>MNNPAIKRIGNHITKSPEDKREYRGLELANGIKVLLISDPTTDKSSAALDVHIGSLSDPPNIAGLSHFLQHMLFLGTKKYPKENEYSQFLSEHAGSSNAFTSGEHTNYYFDVSHEHLEGALDRFAQFFLSPLFDESAKDREVNAVDSEHEKNVMNDAWRLFQLEKATGNPKHPFSKFGTGNKYTLETRPNQEGIDVRQELLKFHSAYYSSNLMAVVVLGRESLDDLTNLVVKLFSEVENKNVPLPEFPEHPFQEEHLKQLYKIVPIKDIRNLYVTFPIPDLQKYYKSNPGHYLGHLIGHEGPGSLLSELKSKGWVNTLVGGQKEGARGFMFFIINVDLTEEGLLHVEDIILHMFQYIQKLRAEGPQEWVFQELKDLNAVAFRFKDKERPRGYTSKIAGILHYYPLEEVLTAEYLLEEFRPDLIEMVLDKLRPENVRVAIVSKSFEGKTDRTEEWYGTQYKQEAIPDEVIKKWQNADLNGKFKLPTKNEFIPTNFEILPLEKEATPYPALIKDTAMSKLWFKQDDKFFLPKANLNFEFFSPFAYVDPLHSNMAYLYLELLKDSLNEYAYAAELAGLSYDLQNTIYGMYLSVKGYNDKQPILLKKIIEKMATFEIDEKRFEIIKEAYMRSLNNFRAEQPHQHAMYYLRLLMTEVAW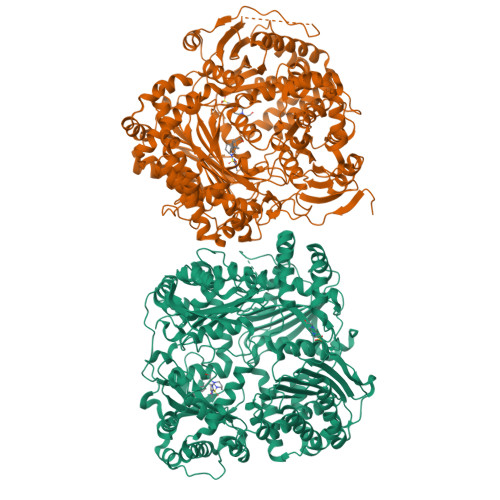TKDELKEALDDVTLPRLKAFIPQLLSRLHIEALLHGNITKQAALGIMQMVEDTLIEHAHTKPLLPSQLVRYREVQLPDRGWFVYQQRNEVHNNSGIEIYYQTDMQSTSENMFLELFAQIISEPAFNTLRTKEQLGYIVFSGPRRANGIQGLRFIIQSEKPPHYLESRVEAFLITMEKSIEDMTEEAFQKHIQALAIRRLDKPKKLSAESAKYWGEIISQQYNFDRDNTEVAYLKTLTKEDIIKFYKEMLAVDAPRRHKVSVHVLAREMDSNPVVGEFPAQNDINLSQAPALPQPEVIQNMTEFKRGLPLFPLVKPHINFMAAKL[2x]> MNKLACLSGRFGRPGIVFIGVAALWWLITRYGAYLGAETRRDQILLLILLSLGVLFVCYLPVMKKYVQELTYRRRARKEQRLPDDEERLAQTPPRYVTVQDIRHTLRRQYGRFWGRKIRILLITGTASEVELLTPGLTEQFWQEEQGTLLLWGGDPSQPENADWLAALRRLRYRPADGIVWVTSGLSETLSAPLTEDALDRVSRAVSSCCERLGWRLPLYVWSLQESPDERGRITQPVGCLLPAECSSDK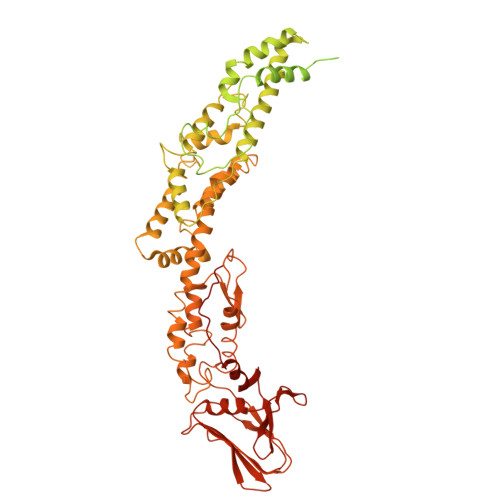LKAQLQAMLPGLVAQGIQQICCAPRYYFLLSLAERFRRNIDAVVEPLSVLLRPYRQLLLAGIVFSPATVGGERSVRHRWRMDNRWEALPETVQQLPVRLQPSRTGHNWRRSLAVMAAILMMAQGTGMVVSFLANRSLVAEVQEQIRPAQNQQLSPAERLQALLNLQKSLARLQYREEHGAPWYLRAGMNQNADLLAVVMPLYAQNAHLLLRDAAAAHLEQQLRTFIRLPPDSPQRGKMAKAAYDQLRLYLMLAQPQHMEPAWFSRTLMREWPQRDGVSAVFWQANGPTLLAYYASGIITHPQWKLTADEELVSQSRTLLLRHLGTQNSDAMLYQKMLARVAHQFADMRLTDMTGDTDVSRLFFTDEVVPGMFTRQAWEEAVLPSIDTVINERREEMDWVLTDGRQKAPSPVSPEALRQRLTTRYFADFGNAWLNFLNSLHLRKAQTLSDVTEQLTLMADVRQSPLVALMNTLAVQGCTGQPREAVTDSLVKSARNLLSQEKQPVAVPESRLHGPLATTFGPVLALMDNQNNSADMLNLQTYLTRVTQVRLRLQQIAGSSDPQAMMQLLAQTVLQGKSVDLTDTRDYGSLTAAGLGQEWYGFGQTVFVRPMEQAWQQVLTPAAESLNARWRTAVVDGWNNAFSGRYPFKNVSSDASLPLLAKYLNTDTGRIARFLQNNLSGVLHREGSRWVPDTINTRGLTFNPAFLKAINTLSEIADVAFTTGNAGLHFELRPGTAAGVMQTTLITDNQKLIYVNQMPVWKRFTWPADTEAPGASLSWVSTQAGTRQYADLPGSWGLIRLLEMARRKAAPGVASGWSLSWQAQDGRMLNYTLRTEAGEGPLVLLKLRNFVLPETVFELSGTSAFTGNDEDAGDTVEETD Hydroxynitrile lyases (HNLs) catalyze the enantioselective interconversion of cyanohydrins and aldehydes/ketones. One example of an HNL with an α/β-hydrolase fold is the hydroxynitrile lyase from the Pará rubber tree Hevea brasiliensis (HbHNL). HNLs occur in at least four protein folds; this paper focuses on HNLs with an α/β-hydrolase fold. This fold consists of eight β-strands connected by α-helices and contains a catalytic triad, typically Ser–His–Asp. HbHNL and SABP2 also use the same Ser–His–Asp catalytic triad even though the catalytic mechanisms of ester hydrolysis and cyanohydrin cleavage differ significantly.

We report a 1.99 Å resolution crystal structure of HNL6V, an engineered variant of hydroxynitrile lyase from Hevea brasiliensis (HbHNL) containing seven amino-acid substitutions (T11G, E79H, C81L, H103V, N104A, G176S and K236M). Six of the seven substitutions replace residues in and around the active site with a corresponding residue from SABP2 (Thr11Gly, Glu79His, Cys81Leu, Asn104Ala, Gly176Ser and Lys236Met). The seventh substitution, His103Val, introduces an amino acid similar to the leucine in SABP2. The harvested crystal belonged to space group C2221, with unit-cell parameters a = 47.05, b = 106.38, c = 128.40 Å and one molecule per asymmetric unit. As this electron density near the catalytic serine Oγ remains unmodeled, this model should be considered a putative structure. The structure reveals that HNL6V maintains the characteristic α/β-hydrolase fold while exhibiting systematic shifts in backbone and catalytic atom positions. Compared with wild-type HbHNL, the Cα positions in HNL6V differ by a mean of 0.2 ± 0.1 Å, representing a statistically significant displacement. Importantly, the catalytic triad and oxyanion-hole atoms have moved 0.2–0.8 Å closer to their corresponding positions in SABP2, although they remain 0.3–1.1 Å from fully achieving the configuration of SABP2. Although HNL6V contains the Cys81Leu substitution, the side chain of the leucine still points in the same direction as the cysteine in HbHNL.

> MAFAHFVLIHGICHGAWIWHKLKPLLEALGHKVTALDLAASGVDPRQIEEIGSFDEYSEPLLTFLEALPPGEKVILVGHSLGGLNIAIAADKYCEKIAAAVFVASVLPDTEHCPSYVVDKLMEVFPDWKDTTYFTYTKDGKEITGLKLGFTLLRENLYTLCGPEEYELAKMLTRKSSLFQNILAKRPFFTKEGYGSIKKIYVWTDQDEIFLPEFQLWQIENYKPDKVYKVEGGDHMLQLTKTKEIAEILQEVADTYNLEHHHHHH> XSLSDKDKAAVRALWSKIGKSADAIGNDALSRMIVVYPQTKTYFSHWPDVTPGSPHIKAHGKKVMGGIALAVSKIDDLKTGLMELSEQHAYKLRVDPANFKILNHCILVVISTMFPKEFTPEAHVSLDKFLSGVALALAERYR;> VEWTDKERSIISDIFSHMDYDDIGPKALSRCLIVYPWTQRHFSGFGNLYNAEAIIGNANVAAHGIKVLHGLDRGVKNMDNIAATYADL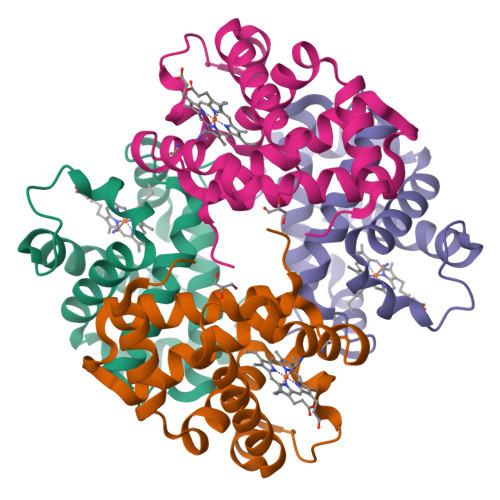STLHSEKLHVDPDNFKLLSDCITIVLAAKMGHAFTAETQGAFQKFLAVVVSALGKQYH sulfuric diamide | H4 N2 O2 S | 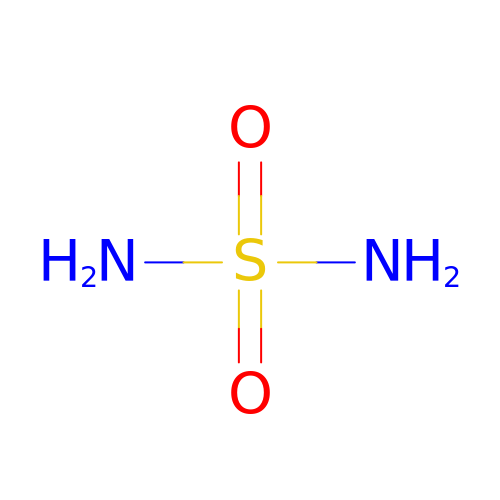NVBFHJWHLNUMCV-UHFFFAOYSA-N> TDTTNSIKHVISPLARQTLQDRDLTRPVAGKRPIRLLPWLQVVKIGGRVMDRGADAILPLVEELRKLLPEHRLLILTGAGVRARHVFSVGLDLGLPVGSLAPLAASEA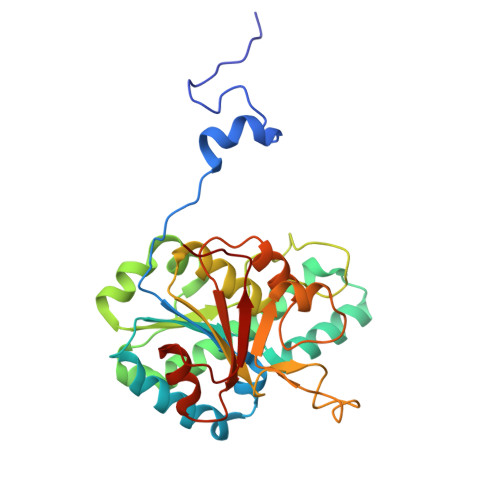GQNGHILAAMLASEGVSYVEHPTVADQLAIHLSATRAVVGSAFPPYHHHEFPGSRIPPHRADTGAFLLADAFGAAGLTIVENVDGIYTADPNGPDRGQARFLPETSATDLAKSEGPLPVDRALLDVMATARHIERVQVVNGLVPGRLTAALRGEHVGTLIRTGVRPA>MDLSELERDNTGRCRLSSPVPAVCRKEPCVLGVAEAGRGPVLGPMVYAICYCPLPRLADLEALKVADSKTLLESERERLFAKMEDTDFVGWALDVLSPNLISTSMLGRVKYNLNSLSHDTATGLIQYALDQGVNVTQVFVDTVGMPETYQARLQQSFPGIEVTVKAKAAALYPVVSAASICAKVARDQAVKKWQFVEKLQDLDTDYGSGYPNDPKTKAWLKEHVEPVFGFPQFVRFSWRTAQTILEKEAEDVIWEDSASENQEGLRKITSYFLNEGSQARPRSSHRYFLERGLESATSL[2x];>GPLGSPEFPGRLAAGVDCGDGVGARQHVFLVSEYLKDASKKMKNGLMFVKLVNPCSGEGAIYLFNMCLQQLFEVKVFKEKHHSWFINQSVQSGGLLHFATPVDPLFLLLHYLIKADKEGKFQPLDQVVVDNVFPNCILLLKLPGLEKLLHHVTEEKGNPEIDNKKYYKYSKEKTLKWLEKKVNQTVAALKTNNVNVSSRVQSTAFFSGDQASTDKEEDYIRYAHGL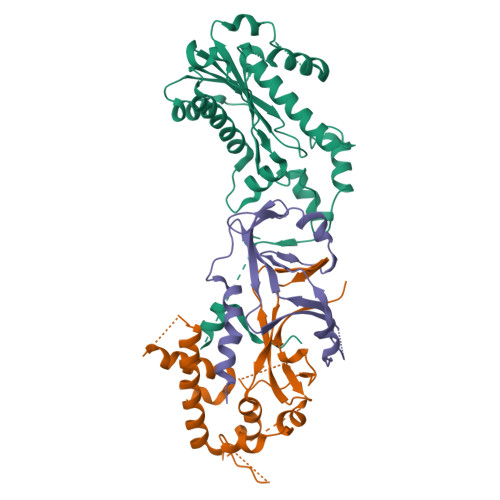ISDYIPKELSD[2x];>MESGDEAAIERHRVHLRSATLRDAVPATLHLLPCEVAVDGPAPVGRFFTPAIRQGPEGLEVSFRGRCLRGEEVAVPPGLVGYVMVTEEKKVSMGKPDPLRDSGTDDQEEEPLERDFDRFIGATANFSRFTLWGLETIPGPDAKVRGALTWPSLAAAIHAQVPED[2x]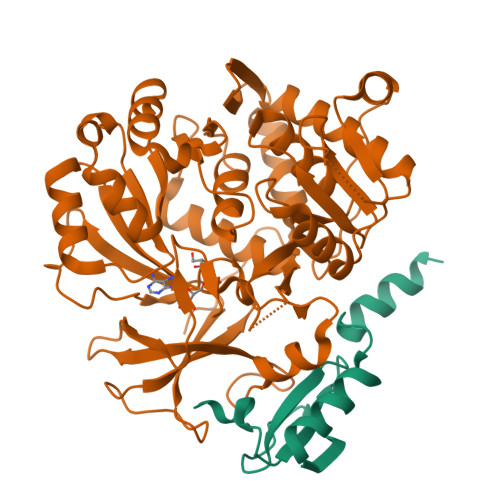> AMADIGSMTNPFDDDEGVFLVLVNDEDQYSLWPEFAEVPQGWRTVFGPTSRAAALDYINTHWTDLRPRSLREAMEAHSTAG;> GSHMASMTGGQQMGRGSEFDSERPLCAFDLLGDAERAALAAHNATRHPLAEHTLTALVDAAAHTHADRVALIADGIRLTYREVHDRAGRLAALLAERGVAPGDVVAVALPRSADLVIALLGVLRAGAAYLPLDVDHPPARLAAMVERARAGTVVTCQGALPRLGDRLPGTVVVDDAATRDRLAGLEPLPTRDVHPDQLAYTIFTSGSTGEPKGVGVAHRAIANRLQWMQHTYRLTPEDRVAQKTPVGFDVSVWEFFWPLITGATLVVARPGGHRDPAYLAALFAEHKVTVCHFVPSLLRVFLNEPTARRATALRQVIVSGEALDADLARAWARTLPQARLDNLYGPTEAAVDVTSHPVCGAGTEPVRDPVPIGRPVWNTELYVLDSSLRPLPTGAVGELYLGGVQLARGYVGRPGMTASRFVANPFGPPGSRLYRTGDLVRRRADGAVEYLGRVDDQVKINGVRVEPGEVEAVLRAQPGVADAAVAARPAPAGGLRLVGYLVPDGSPPDVDEVRRGLADRLPAAWVPAAFVVVDALPLTVNGKLRRDALPDPDPGPV> MRMTWNFHQYYTNRNDGLMGKLVLTDEEKNNLKALRKIIRLRTRDVFEEAKGIAKAVKKSALTFEIIQEKVSTTQIKHLSDSEQREVAKLIYEMDDDARDEFLGLTPRFWTQGSFQYDTLNRPFQPGQEMDIDDGTYMPMPIFESEPKIGHSLLILLVDASLKSLVAENHGWKFEAKQTCGRIKIEAEKTHIDVPMYAIPKDEFQKKQIALEANRGSGSENVNLALREGDRKWINSDPKIVEDWFNDSCIRIGKHLRKVCRFMKAWRDAQWDVGGPSSISLMAATVNILDSVAHDASDLGETMKIIAKHLPSEFARGVESPDSTDEKPLFPPSYKHGPREMDIMSKLERLPEILSSAESADSK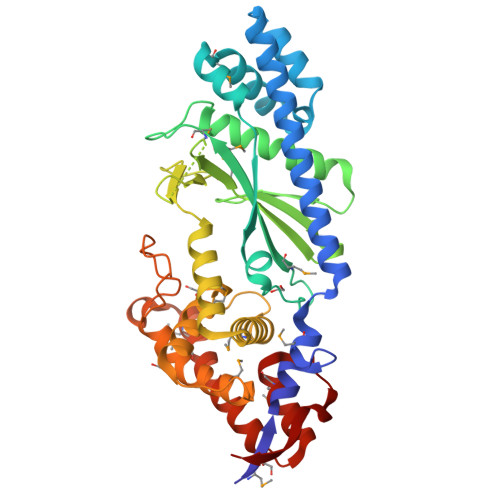SEALKKINMAFGNRVTNSELIVLAKA> MAKGEGAESGSAAGLLPTSILQSTERPAQVKKEPKKKKQQLSICNKLCYAVGGAPYQVTGCALGFFLQIYLLDVAQVGPFSASIILFVGRAWDAITDPLVGFCISKSSWTRLGRLMPWIIFSTPLAVIAYFLIWFVPDFPHGQTYWYLLFYCLFETLVTCFHVPYSALTMFISTEQSERDSATAYRMTVEVLGTVLGTAIQGQIVGQADTPCFQDLNSSTVASQSANHTHGTTSHRETQNAYLLAAGVIASIYVICAVILTLGVREQREPYEAQQSEPMSFFRGLRLVMSHGPYIKLIAGFLFTSLAFMLVEGNFALFCTYTLGFRNEFQNLLLAIMLSATLTIPIWQWFLTRFGKKTAVYVGISSAVPFLILVALMESNLIVTYVVAVAAGIS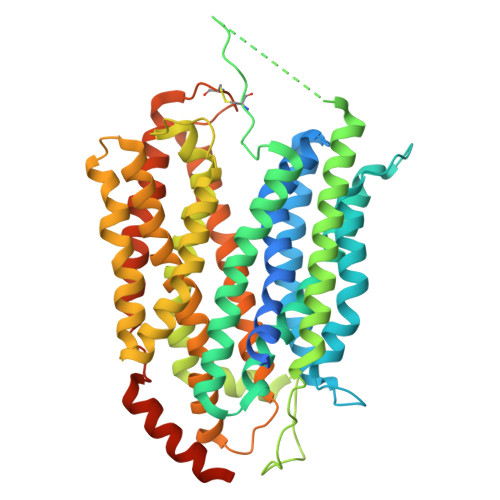VAAAFLLPWSMLPDVIDDFHLKQPHSHGTEPIFFSFYVFFTKFASGVSLGISTLSLDFAGYQTRGCSQPERVKFTLKMLVTMAPIVLILLGLLLFKLYPIDEERRRQNKKALQALRDEASSSGCSETDSTELASIL>[4x]LPNITILATGGTIAGGGDSATKSNYTAGKVGVENLVNAVPQLKDIANVKGEQVVNIGSQDMNDDVWLTLAKKINTDCDKTDGFVITHGTDTMEETAYFLDLTVKCDKPVVMVGAMRPSTSMSADGPFNLYNAVVTAADKASANRGVLVVMNDTVLDGRDVTKTNTTDVATFKSVNYGPLGYIHNGKIDYQRTPARKHTSDTPFDVSKLNELPKVGIVYNYANASDLPAKALVDAGYDGIVSAGVGNGN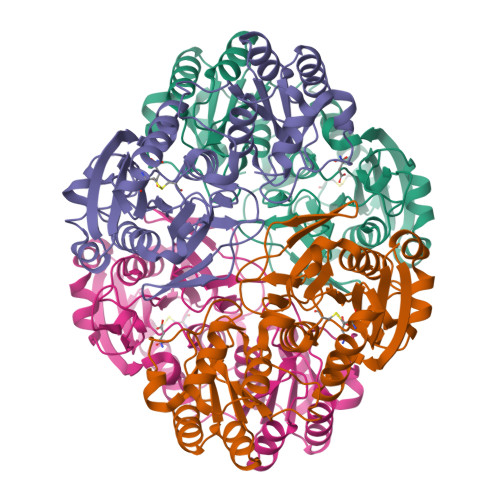LYKTVFDTLATAAKNGTAVVRSSRVPTGATTQDAEVDDAKYGFVASGTLNPQKARVLLQLALTQTKDPQQIQQIFNQY>RICFNHQSSQPQTTKTCSPGESSCYHKQWSDFRGTIIERGCGCPTVKPGIKLSCCES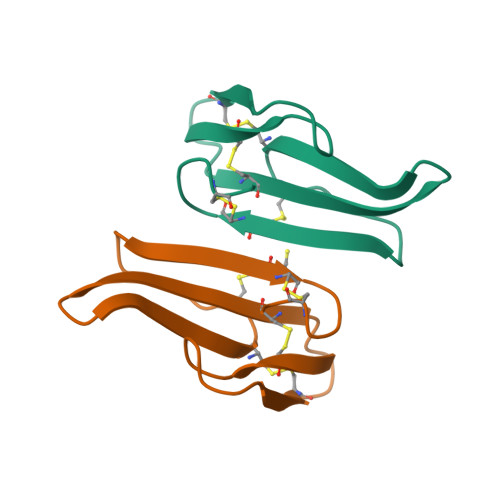EVCNN[2x]> MTVPTNDNREQYAGNGATTVFPYAFRIFESSDLEVYLTDEDGDQALLIEGTDYTVSGAGDEEGGEITFPVSGDPLDDGETLTILRVIDITQETDLKNQGAYYPEVVEDEFDRSRMIDQQQQEQLDRALIKTETGDRWEGQGVPAKNFAMSDPVEDTDLPTVRWTKDYVTQMAEGITGDIGAYTVVAPTSGDEKRLDEWMDDIQRPDDSLVVADGGTEARSLSERFADSASYQDYGIAGDGTTNDTAAFAAL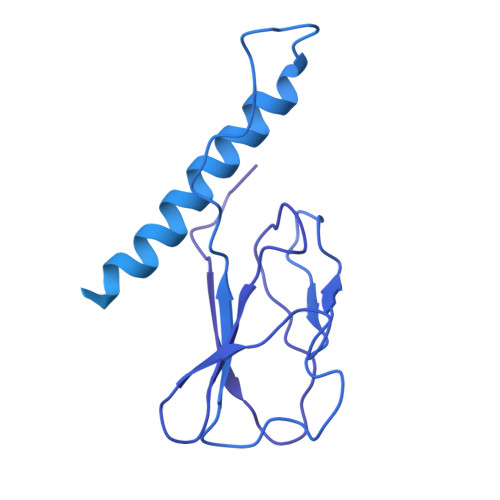ESDRSSDAIELHGNTYLVDEIPNGNAYRDAVWSLDGEDLSISEYGGLVTGTPTTGAFEPAYTGGVNNTPTTSGRTNKHTRAILASQNCRADFARSACVASIYSWAYGNVSGNFASRQSIAGAPQTVNIGSEEGQALGFQSGNYTTQFCRAEGSTTFNIGSDDCAASGAHSGTISSLESYAGRGHDFRGTPVFDDGVLVDITIDDAGAGYVPGSDVMYLQNRQFGNTTDAVITYTVDGTGGVSAITITDGGSGYSGIVAARIDTFGDYSLVMASARSKIEDQFCAAIASDNARVRGRESAVIASDGGVVNEDNSVVIGSVDSTSNGARSGIYTGSGCETTGAGAVVIGGVNAKASNDGAIVMGRGVDSEFARSLVFGDGGSGAAASTAGRKFQVTAAGNVTAAGTITGSTTYADYAEYFENSARGVIPLGVIVTLDGRKVRPASAGDDIIGVVSGTAILAAGDSQFHWGGRYLAGEFGELLYHDVDVDGKIERQPVENPEYDPSVPNVPRSQRPEEWSCIGLVGQLHVRVSSDVAAGDRVAAGDGGIGVPGDNGMICMEIKQAYDSGKGYAVALCLHK5-((3aS,4S,6aR)-2-oxohexahydro-1H-thieno[3,4-d]imidazol-4-yl)-N-((S)-pyrrolidin-3-yl)pentanamide | C14 H24 N4 O2 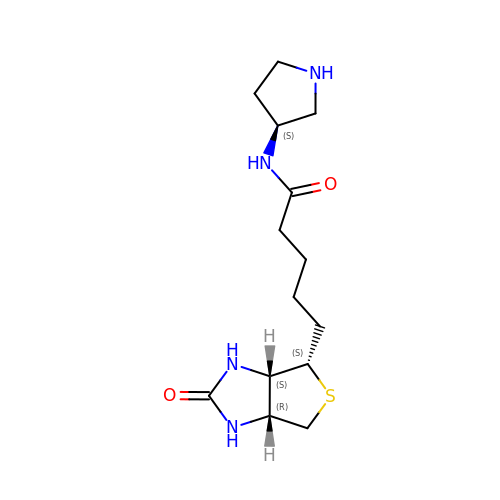S | QSMYOZNFIUDGEL-ZPFDUUQYSA-N>MGSDKIHHHHHHENLYFQGMIESIQELLQKEAQAVLNIPVTDAYEKAVELIVEQIHRKKGKLVTSGMGKAGQIAMNIATTFCSTGIPSVFLHPSEAQHGDLGILQENDLLLLI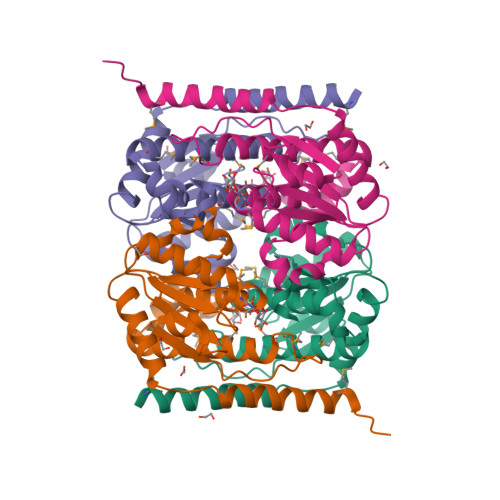SNSGKTREIVELTQLAHNLNPGLKFIVITGNPDSPLASESDVCLSTGHPAEVCTLGMTPTTSTTVMTVIGDILVVQTMKRTEFTIEEYSKRHHGGYLGEKSRKLCVK[4x]Epidemic keratoconjunctivitis (EKC) is a severe ocular infection and is caused by the highly contagious adenoviruses Ad8, Ad19, and Ad37. The initial event leading to EKC is binding of the viruses to glycans that contain sialic acid moieties on epithelial cells in the cornea or conjunctiva through trimeric fiber structures extending from the viral particles. The receptor-binding domain, the fiber knob, is located at the C terminus of each fiber and contains three separate pockets that each can accommodate one sialic acid residue. The crystal structure of the fiber-knob protein shows that the three known sialic acid binding sites are separated by distances of about 10 Å.

Instead we selected the three small and flexible scaffolds tris(2-aminoethyl)amine, 2-(aminomethyl)-2-methyl-1,3-propanediamine, and 2,2-diaminomethyl-1,3-propanediamine for conjugation with the sialic acid derivative 1 through the use of squaric acid chemistry and thus prepared ME0322, ME0323, and ME0324 in modest to good yields. We reasoned that longer flexible spacers would enable all three binding pockets to be occupied simultaneously by one molecule. Only the terminal sialic acid residues of ME0322 are visible in the final electron-density map. We did not observe electron density for the rest of the compound, probably because the flexible linkers do not make defined contacts with the protein. It is, however, likely that all three sialic acids in a fiber knob belong to the same trivalent compound. Analysis of the crystal packing shows that the distances between sialic acid binding sites in different knobs are too large to be bridged by a single ME0322 molecule (data not shown). The binding of all sialic acid residues and their interactions with their respective protein chains are identical to the previously established binding mode between the sialic acid residues of sialyl-α(2,3)-lactose or the GD1a hexasaccharide and the Ad37 fiber knob. The binding was shown to fit to a simple one-to-one binding model, and the calculated Kd value for the interaction of the Ad37 fiber-knob protein with ME0322 was calculated to be 14 μm. Compound ME0322 proved to be very potent and inhibited the infection of HCE cells by Ad37 virions with an IC50 value of 0.38 μm.

>GAMGSWNPKYDTRTLWTTPDTSPNCTIAQDKDSKLTLVLTKCGSQILANVSLIVVAGKYHIINNKTNPKIKSFTIKLLFNKNGVLLDNSNLGKAYWNFRSGNSNVSTAYEKAIGFMPNLVAYPKPSNSKKYARDIVYGTIYLGGKPDQPAVIKTTFNQETGCEYSITFNFSWSKTYENVEFETTSFTFSYIAQE[6x]>RSNVFAVDSQIPTLYMPQYISLSGVMTNDGPDNQAIASFEIRDQYITALNHLVLSLELPEVKGMGRFGYVPYVGYKCINHVSISSCNGVIWEIEGEELYNNCINNTIALKHSGYSSELNDISIGLTPNDTIKEPSTVYVYIKTPFDVEDTFSSLKLSDSKITVTVTFNPVSDIVIRDSSFDFETFNKEFVYVPELSFIGYMVKNVQIKPSFIEKPRRVIGQINQPTATVTEVHAATSLSVYTKPYYGNTDNKFISYPGYSQDEKDYIDAYVSRLLDDLVIVSDGPPTGYPESAEIVEVPEDGIVSIQDADVYVKIDNVPDNMSVYLHTNLLMFGTRKNSFIYNISKKFSAITGTYSDATKRTIFAHISHSINIIDTSIPVSLWTSQRNVYNGDNRSAESKAKDLFINDPFIKGIDFKNKTDIISRLEVRFGNDVLYSENGPISRIYNELLTKSNNGTRTLTFNFTPKIFFRPTTITANVSRGKDKLSVRVVYSTMDVNHPIYYVQKQLVVVCNDLYKVSYDQGVSITKIMG[3x]

In Vaccinia virus (VACV), copies of the double-jelly-roll protein D13 bind to the viral membrane via interaction with its partner protein A17 and assemble into a scaffold surrounding the viral membrane. This process leads to the formation of a spherical immature virion (IV). The 62-kDa D13 protein exists as trimers both in vivo and in vitro, and structures of the recombinantly expressed D13 trimer have been determined by X-ray crystallography. D13 adopts a double-jelly-roll structure composed of 8 antiparallel β-strands.

Furthermore, we expressed and purified mutant protein (D1318-548) with a truncation of 17 N-terminal amino acid residues, including the N-terminal tail α-helix. Our cryo-EM reconstruction of the mutant displayed no significant change from wild-type D13 (wtD13) or D13 with an intact N-terminal His6-tag. This mutant assembled into tubular and spherical structures that exhibit a honeycomb-like lattice under low-salt conditions in a fashion similar to the His6-tagged protein, thereby confirming the essential function of the N-terminal tail helix for D13 self-assembly. 130,384, 173,354 and 156,813 particle images were used to reconstruct the maps shown in a, b, and c, respectively. Their structures reveal that the wild-type trimer has an intact N-terminal tail helix (colored purple), whereas the corresponding density is missing in His6-tagged protein and in the truncation mutant. Reduction of salt concentration to 150 mM leads to aggregation in case of wtD13, to spherical assemblies for His6-tagged D13, or to a mixture of tubular and spherical assemblies for D1318-548.S-TRITYL-L-CYSTEINE 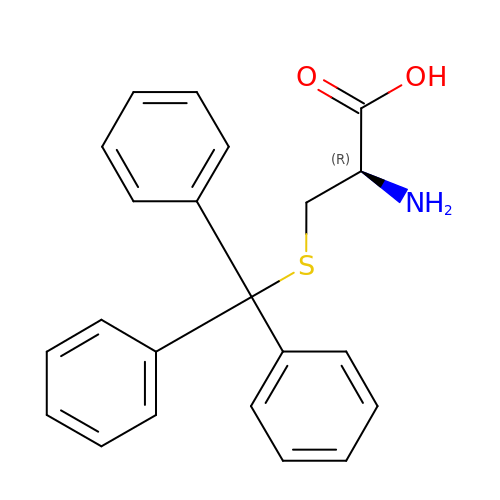| C22 H21 N O2 S | DLMYFMLKORXJPO-FQEVSTJZSA-N> MTAIANRYEFVLLFDVENGNPNGDPDAGNMPRIDPETGHGLVTDVCLKRKIRNHVALTKEGAERFNIYIQEKAILNETHERAYTACDLKPEPKKLPKKVEDAKRVTDWMCTNFYDIRTFGAVMTTEVNCGQVRGPVQMAFARSVEPVVPQEVSITRMAVTTKAEAEKQQGDNRTMGRKHIVPYGLYVAHGFISAPLA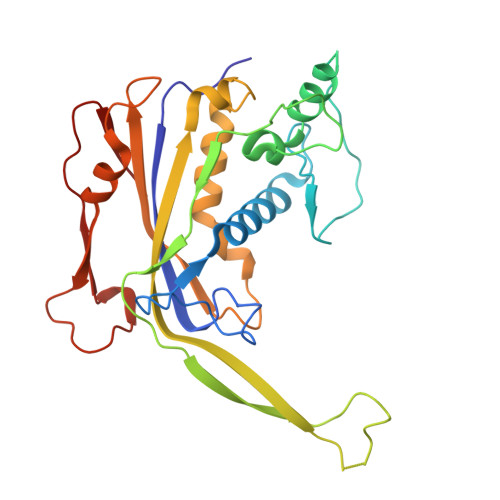EKTGFSDEDLTLFWDALVNMFEHDRSAARGLMSSRKLIVFKHQNRLGNAPAHKLFDLVKVSRAEGSSGPARSFADYAVTVGQAPEGVEVKEML(2-methylquinolin-4-yl)methanol | C11 H11 N O | 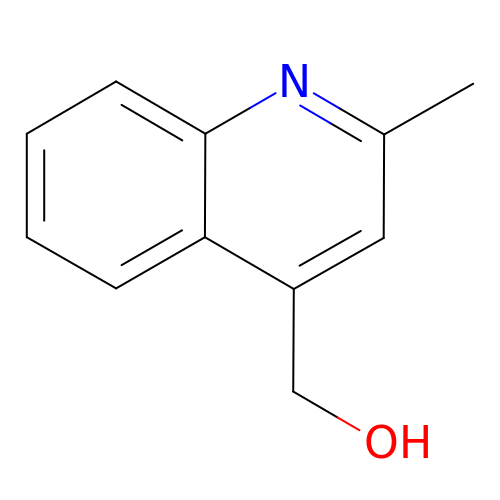MNDWQNXETQDJMZ-UHFFFAOYSA-N> NIPAGIIPTGNVLSTIEVCAHRCIFDFFKQIRSDDNSLYSAQFDILLGTYCNTLNFVRFLELGLSVACICTKFPELAYVRDGVIQFEVQQPMIARDGPHPVDQPVHNYMVKRIHKRSLSAAFAIASEALSLLSNTYVDGTEIDSSLRIRAIQQMARNLRTVSDSFERGTADQLLGVLLEKAPPLSLLSPINKFQPEGHLNRVARAALLSDLKRRVCADMFFMTRHAREPRLISAYLSDMVSCTQPSVMVSRITHTNTRGRQVDGVLVTTATLKRQLLQGILQIDDTAADVPVTYGEMVLQGTNLVTALVMGKAVRGMDDVARHLLDITDPNTLNIPSIPPQSNSDSTTAGLPVNARVPADLVIVGDKLVFLEALERRVYQATRVAYPLIGNIDITFIMPMGVFQANSMDRYTRHAGDFSTVSEQDPRQFPPQGIFFYNKDGILTQLTLRDAMGTICHSSLLDVEATLVALRQQHLDRQCYFGVYVAEGTEDTLDVQMGRFMETWADMMPHHPHWVNEHLTILQFIAPSNPRLRFELNPAFDFFVAPGDVDLPGPQRPPEAMPTVNATLRIINGNIPVPLCPISFRDCRGTQLGLGRHTMTPATIKAVKDTFEDRAYPTIFYMLEAVIHGNERNFCALLRLLTQCIRGYWEQSHRVAFVNNFHMLMYITTYLGNGELPEVCINIYRDLLQHVRALRQTITDFTIQGEGHNGETSEALNNILTDDTFIAPILWDCDALIYRDEAARDRLPAIRVSGRNGYQALHFVDMAGHNFQRRDNVLIHGRPVRGDTGQAIPITPHHDREWGILSKIYYYIVIPAFSRGSCCTMGVRYDRLYPALQAVIVPEIPADEEAPTTPEDPRHPLHAHQLVPNSLNVYFHNAHLTVDGDALLTLQELMGDMAERTTAILVSSAPDAGAATATTRNMRIYDGALYHGLIMMAYQAYDETIATGTFFYPVPVNPLFACPEHLASLRGMTNARRVLAKMVPPIPPFLGANHHATIRQPVAYHVTHSKSDFNTLTYSLLGGYFKFTPISLTHQLRTGFHPGIAFTVVRQDRFATEQLLYAERASESYFVGQIQVHHHDAIGGVNFTLTQPRAHVDLGVGYTAVCATAALRCPLTDMGNTAQNLFFSRGGVPMLHDNVTESLRRITASGGRLNPTEPLPIFGGLRPATSAGIARGQASVCEFVAMPVSTDLQYFRTACNPRGRASGMLYMGDRDADIEAIMFDHTQSDVAYTDRATLNPWASQKHSYGDRLYNGTYNLTGASPIYSPCFKFFTPAEVNTNCNTLDRLLMEAKAVASQSSTDTEYQFKRPPGSTEMTQDPCGLFQEAYPPLCSSDAAMLRTAHAGETGADE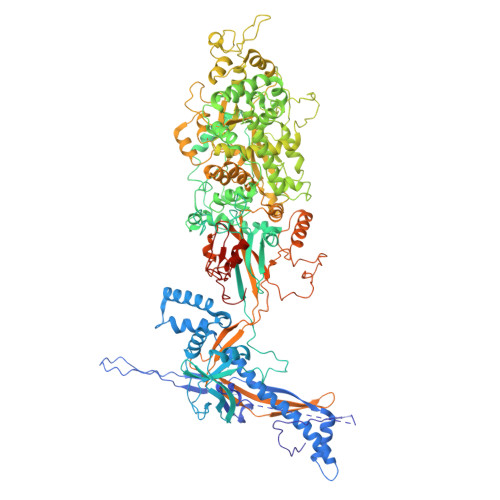VHLAQYLIRDASPLRGCLPL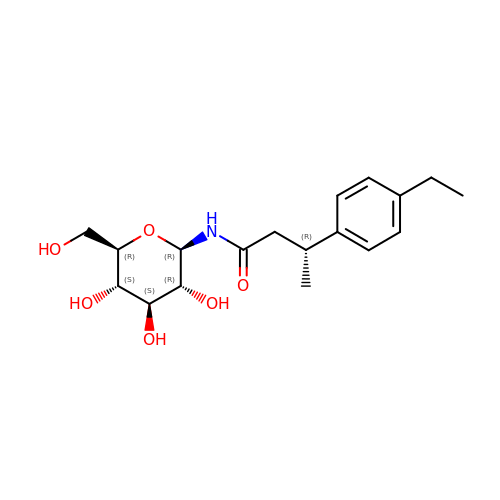N-[(3R)-3-(4-ethylphenyl)butanoyl]-beta-D-glucopyranosylamine | C18 H27 N O6 | HOHFTRIQTPLVFO-JJLIPNPMSA-N> GAMGMSEEELEQDELDGADEDDGEELAAADDGEADSGD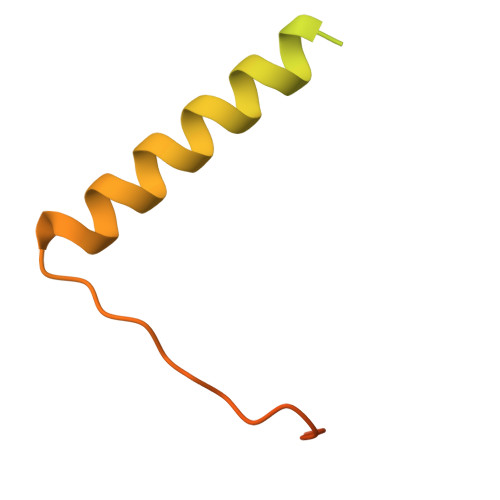GDEAPAPGKKAKAAVVEEELPSVEAKQKERDALAKAMEEFLSRGGKVQEIEPNVVADPPKKPDSKYGSRPI> GPMVLQAQE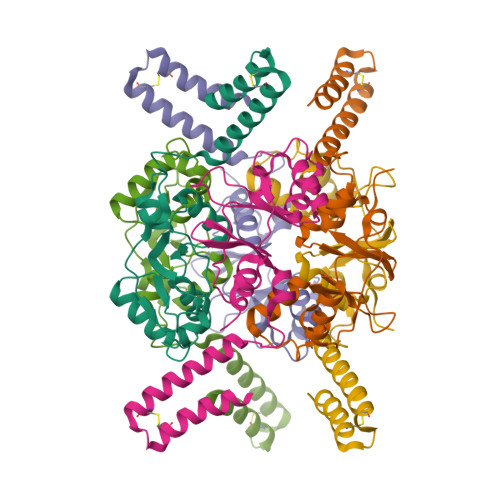IMTQNVVTIRGSATVADAVKLMKEKKLRGLIVEPRHEQDPYGIVTETDIVYKVAAFGHDPKTMRVYEIMAKPCVVVNPELGVEYVARLFAQTRIRRAPVIQGKTLLGIISVSDILFKSDFVEKPKRLFIEDEIEAAREDARAICAAKGETSPDCAAAWDVVEELQAEASHQRAKKQGSNSFQAYCEANPDALECRIYDD> MRSNSQGLSLTDSVYERLLSERIIFLGSEVNDEIANRLCAQILLLAAEDASKDISLYINSPGGSISAGMAIYDTMVLAPCDIATYAMGMAASMGEFLLAAGTKGKRYALPHARILMHQPLGGVTGSAADIAIQAEQFAVI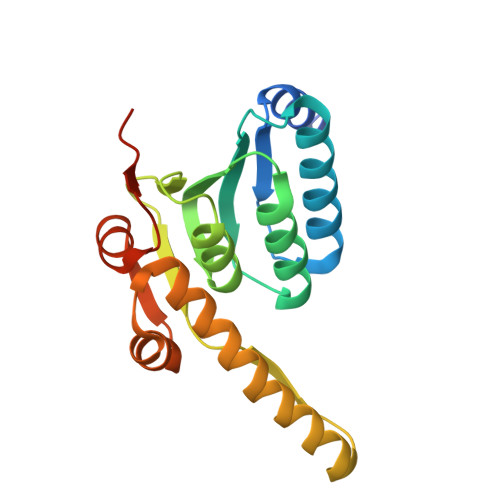KKEMFRLNAEFTGQPIERIEADSDRDRWFTAAEALEYGFVDHIITRAHVNGEAQ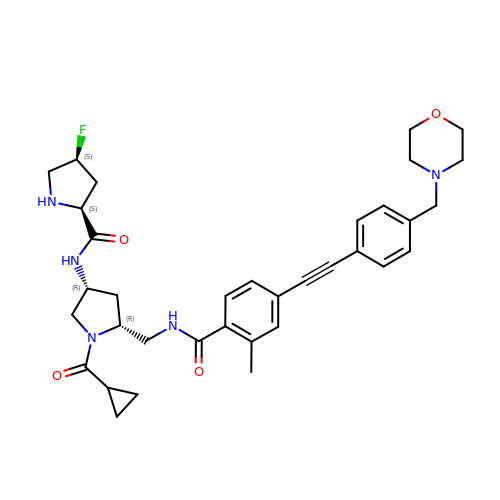(2S,4S)-N-[(3R,5R)-1-cyclopropylcarbonyl-5-[[[2-methyl-4-[2-[4-(morpholin-4-ylmethyl)phenyl]ethynyl]phenyl]carbonylamino]methyl]pyrrolidin-3-yl]-4-fluoranyl-pyrrolidine-2-carboxamide | C35 H42 F N5 O4 | VANITAVOZBNWHX-TWXNZYBRSA-N2-amino-N-(furan-2-ylmethyl)-4-oxo-3,4-dihydropteridine-7-carboxamide | C12 H10 N6 O3 | 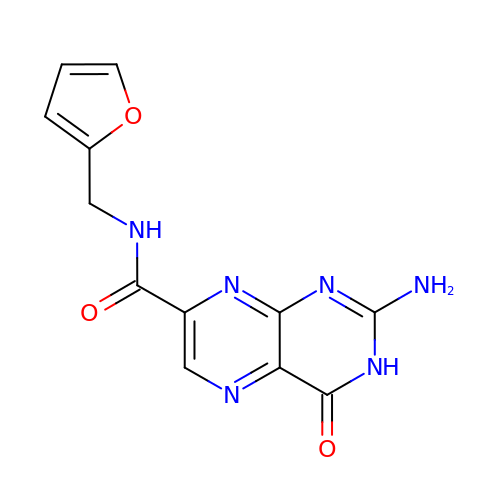UUEDARIHQQJVFX-UHFFFAOYSA-N>[2x]MNTFDKHDLSGFVGKHLVYTYDNGWNYEIYVKNDNTIDYRIHSGLVGNRWVKDQEAYIVRVGESIYKISWTEPTGTDVSLIVNLGD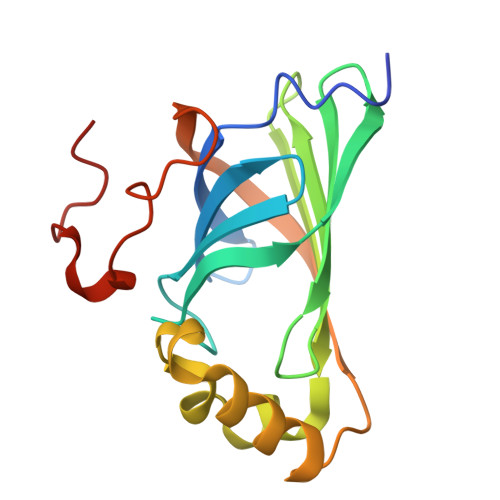SLFHGTIFFPRWVMNNPEPTVCFQNDHIPLMNSYREAGPAYPTEVIDEFATITFVRDCGANNESVIACAASELPKNFPDNLK> QLDKKYKHAGDFGISDTKKNRETLTKFRDAIEEHLSDKDTVEKGTYRREKGSKVYFNPNTMNVVIIKSNGEFLSGWKINPDADNGRIYLE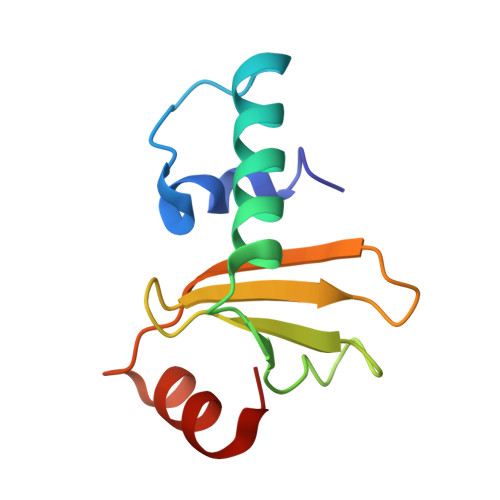TGEL> GEFSSPPKWMAEIERDD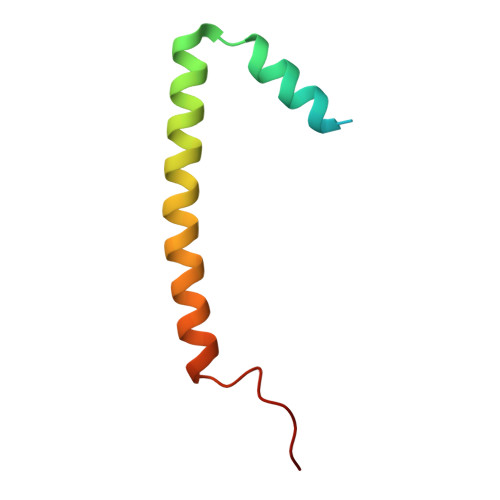IDMLKELGSLTTANLMEKVRGLQNLAYQLGLDESREMTRGKFLNILEKPKK(2S)-4-(4-fluorobenzyl)-N-(2-sulfanylethyl)piperazine-2-carboxamide | C14 H20 F N3 O S | 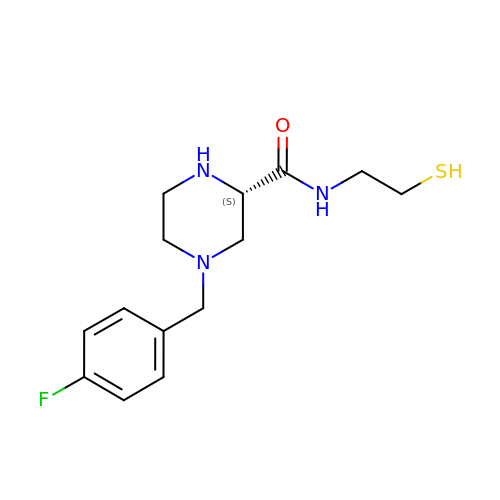CEXXKSSFAKABEN-ZDUSSCGKSA-N> ANLNGTLMQYFEWYMPNDGQHWKRLQNDSAYLAEHGITAVWIPPAYKGTSQADVGYGAYDLYDLGEFHQKGTVRTKYGTKGELQSAIKSLHSRDINVYGDVVINHKGGADATEDVTAVEVDPADRNRVISGEHLIKAWTHFHFPGRGSTYSDFKWHWYHFDGTDWDESRKLNRIYKFQGKAWDWEVSNE;> NGNYDYLMYADIDYDHPDVAAEIKRWGTWYANELQLDGFRLDAVKHIKFSFLRDWVNHVREKTGKEMFTVAEYWQNDLGALENYLNKTNFNHSVFDVPLHYQFHAASTQGGGYDMRKLLNSTVVSKHPLKAVTFVDNHDTQPGQSLESTVQTWFKPLAYAFILTRESGYPQVFYGDMYGTKGDSQREIPALKHKIEPILKARKQYAYGAQHDYFDHHDIVGWT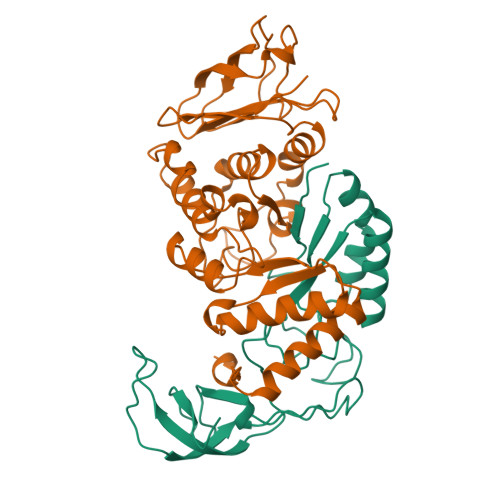REGDSSVANSGLAALITDGPGGAKRMYVGRQNAGETWHDITGNRSEPVVINSEGWGEFHVNGGSVSIYVQR> MEPLKVEKFATANRGNGLRAVTPLRPGELLFRSDPLAYTVCKGSRGVVCDRCLLGKEKLMRCSQCRVAKYCSAKCQKKAWPDHKRECKCLKSCKPRYPPDSVRLLGRVVFKLMDGAPSESEKLYSFYDLESNINKLTEDKKEGLRQLVMTFQHFMREEIQDASQLPPAFDLFEAFAKVICNSFTICNAEMQEVGVGLYPSISLLNHSCDPNCSIVFNGPHLLLRAVRDIEVGEELTICYLDMLMTSEERRKQLRDQYCFECDCFRCQTQDKDADMLTGDEQVWKEVQESLKKIEELKAHWKWEQVLAMCQAIISSNSERLPDINIYQLKVLDCAMDACINLGLLEEALF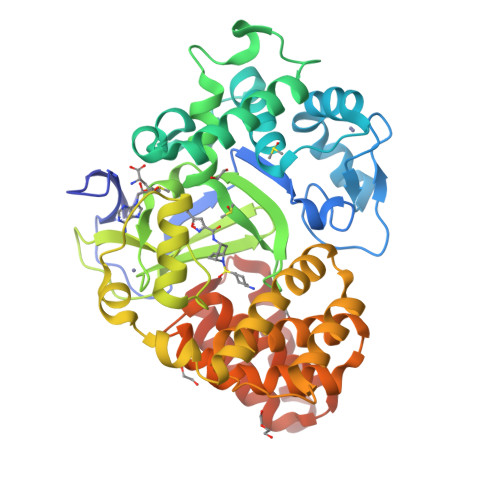YGTRTMEPYRIFFPGSHPVRGVQVMKVGKLQLHQGMFPQAMKNLRLAFDIMRVTHGREHSLIEDLILLLEECDANIRAS2,2-difluoro-3,3-dihydroxybutanedioic acid | C4 H4 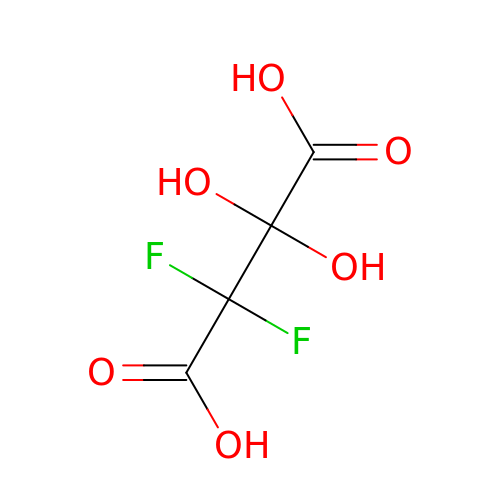F2 O6 | PNUBNHHFDUCRFW-UHFFFAOYSA-N>[2x]MGSSHHHHHHSSENLYFQGHMRLSREDLLERSEVADELLTALLKA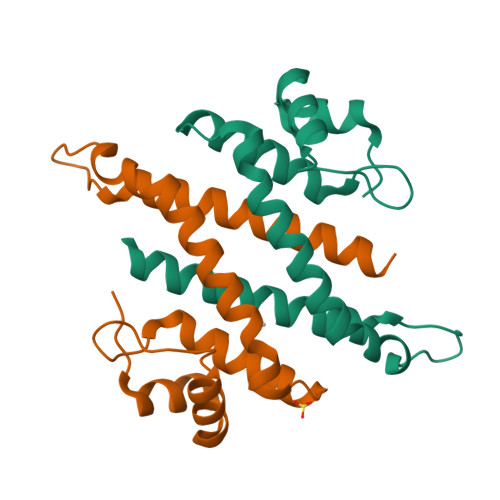GVITTGPGGFFDEHAVVILQCARALAEYGVEPRHLRAFRSAADRQSDLIAQIAGPLVKAGKAGARDRADDLAREVAALAITLHTSLIKSAVRDVLHR> MEYEWKPDEQGLQQILQLLKESQSPDTTIQRTVQQKLEQLNQYPDFNNYLIFVLTKLKSEDEPTRSLSGLILKNNVKAHFQNFPNGVTDFIKSECLNNIGDSSPLIRATVGILITTIASKGELQNWPDLLPKLCSLLDSEDYNTCEGAFGALQKICEDSAEILDSDVLDRPLNIMIPKFLQFFKHSSPKIRSHAVACVNQFIISRTQALMLHIDSFIENLFALAGDEEPEVRKNVCRALVMLLEVRMDRLLPHMHNIVEYMLQRTQDQDENVALEACEFWLTLAEQPICKDVLVRHLPKLIPVLVNGMKYSDIDIILLKGDVEEDETIPDSEQDIGGSGGSGDTISDWNLRKCSAAALDVLANVYRDELLPHILPLLKELLFHHEWVVKESGILVLGAIAEGCMQGMIPYLPELIPHLIQCLSDKKALVRSITCWTLSRYAHWVVSQPPDTYLKPL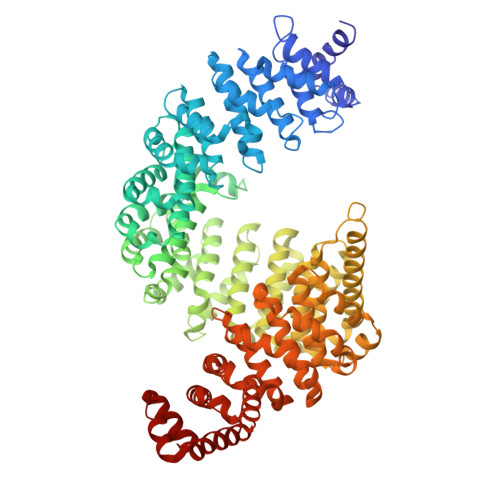MTELLKRILDSNKRVQEAACSAFATLEEEACTELVPYLAYILDTLVFAFSKYQHKNLLILYDAIGTLADSVGHHLNKPEYIQMLMPPLIQKWNMLKDEDKDLFPLLECLSSVATALQSGFLPYCEPVYQRCVNLVQKTLAQAMLNNAQPDQYEAPDKDFMIVALDLLSGLAEGLGGNIEQLVARSNILTLMYQCMQDKMPEVRQSSFALLGDLTKACFQHVKPCIADFMPILGTNLNPEFISVCNNATWAIGEISIQMGIEMQPYIPMVLHQLVEIINRPNTPKTLLENTAITIGRLGYVCPQEVAPMLQQFIRPWCTSLRNIRDNEEKDSAFRGICTMISVNPSGVIQDFIFFCDAVASWINPKDDLRDMFCKILHGFKNQVGDENWRRFSDQFPLPLKERLAAFYGV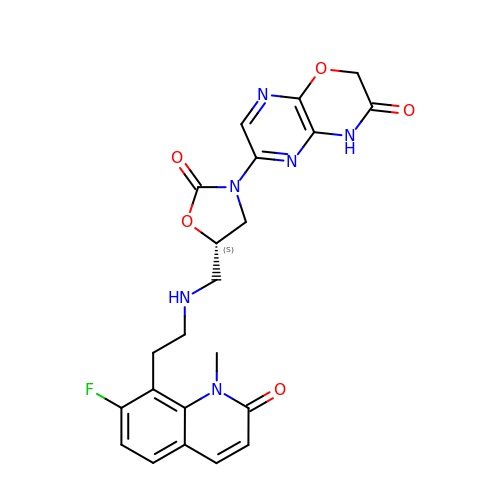6-[(5S)-5-[[[2-(7-Fluoro-1,2-dihydro-1-methyl-2-oxo-8-quinolinyl)ethyl]amino]methyl]-2-oxo-3-oxazolidinyl]-2H-pyrazino[2,3-b]-1,4-oxazin-3(4H)-one | C22 H21 F N6 O5 | MKICNOUBIXXGPQ-UHFFFAOYSA-N>[3x]MSELLVYMNGEFVPESQAKVSVFDHGFLYGDGVFEGIRAYNGKVFKLYEHIDRLYDCARVIDLKIPLSKEEFAEAILETLRRNNLRDAYIRPIVTRGAGDLGLDPRKCPSPNVIIITKPWGKLYGDLYEKGLKAITVAIRRNAIDSLPPNIKSLNYLNNILAKIEANAKGGDEAIFLDHNGYISEGSGDNIFIVKNGTITTPPTLNNLKGITRQVVIELINELEIPFREANIGLFDLYS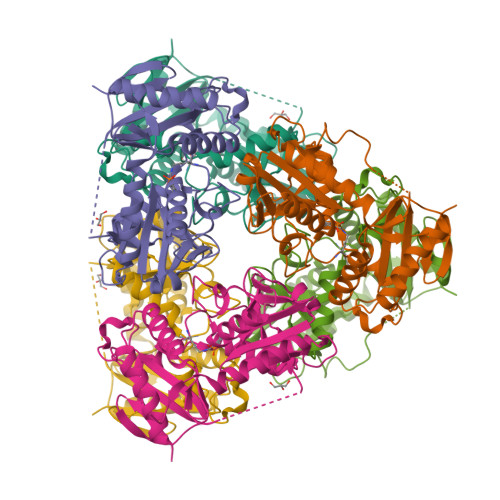ADEIFVTGTAAEIAPVTYIDGRTVGNGKPGKVTKMLMEKFRERTENEGVEIYR>[2x]MRGSHHHHHHGSLRSSRKKMSAASSIFDFEVLDADHKPYNLVQHKGSPLLIYNVASKCG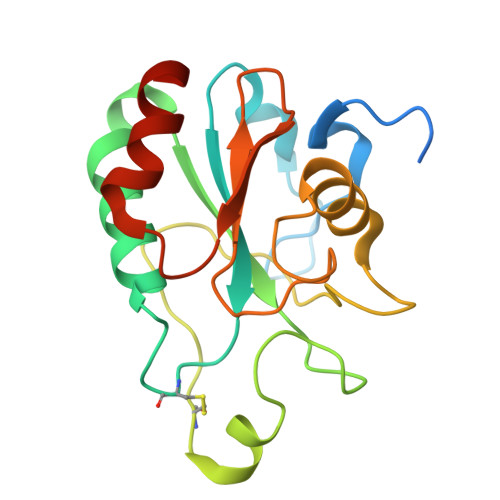YTKGGYETATTLYNKYKSQGFTVLAFPSNQFGGQEPGNEEEIKEFVCTKFKAEFPIMAKINVNGENAHPLYEYMKKTKPGILATKAIKWNFTSFLIDRDGVPVERFSPGASVKDIEEKLIPLLGSARL> RVLQLKLGNSAIVTQEAANYCCAYGEWPNYLPDHEAVAIDKPTQPETATDRFYTLRSVKWEAGSTGWWWKLPDALNNIGMFGQNVQHHYLYRSGFLIHVQCNATKFHQGALLVVAIPEHQRGAHNTNTSPGFDDIMKGEEGGTFNHPYVLDDGTSLACATIFPHQWINLRTNNSATIVLPWMNAAPMDFPLRH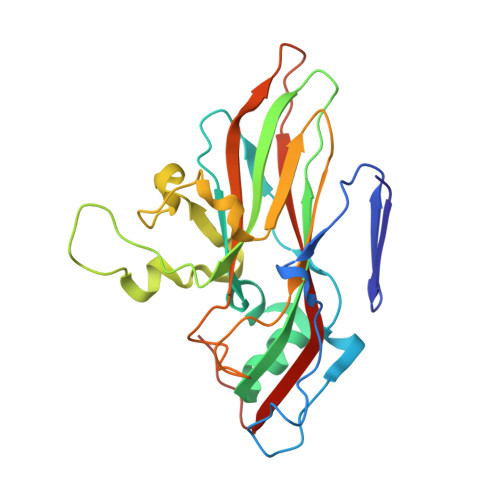NQWTLAIIPVVPLGTRTMSSMVPITVSIAPMCCEFNGLRHAITQ>MAGARQELDTFTRGLKGLDGQFSQRVTDANGRVKENSSGRVALATPRQFRWEYAKPYKQLIVADGKKVWVFDPDLEQVTVRAQGSEEQNSPLVALIDPTRLDKQYDVSEEAAPRDGLQWLSLTPKVDTDASFQMASLGFGKDGLAKMEVVDAVGQRTAISFSGWKRNPAFAADTFRYTPGKGVDVVGDAQAENLYFQSHHHHHH[2x];>MVSVPRGQGGAAPAVVGQVSESARQAEAARQAWLQAHPAWSFQGRVAISKGRDGGSGRLDWQQDGPRYHVQLSAPVTRQSWVLTGDTTTGAGRLEGLDG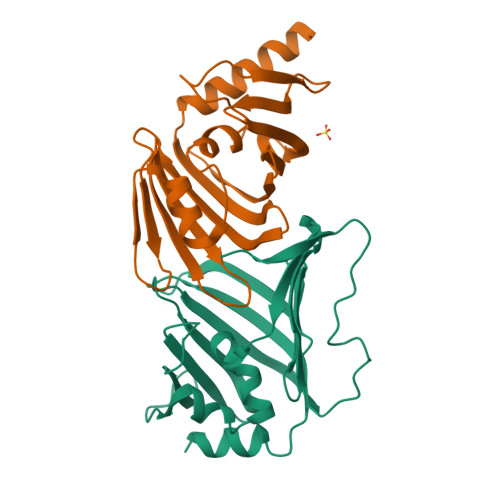GPRAGADAEQVLLEATGWTIPVNQMPDWVRALRIADAGAARVDLDEHGRPRTVQQDGWTIDFLEWTPASAAQPELPRRIEARNGDAKVRLLVDQWTLSPAENLYFQSHHHHHH[2x]>MRGSHHHHHHGIDHMPVEGSEEDKSQTGVNRASKGGLIYGNYLHLEKVLNAQELQSETKGNKIHDEHLFIITHQAYELWFKQILWELDSVREIFQNGHVRDERNMLKVVSRMHRVSVILKLLVQQFSILETMTALDFNDFREYLSPASGFQSLQFRLLENKIGVLQNMRVPYNRRHYRDNFKGEENELLLKSEQEKTLLELVEAWLERTPGLEPHGFNFWGKLEKNITRGLEEEFIRIQAKEESEEKEEQVAEFQKQKEVLLSLFDEKRHEHLLSKGERRLSYRALQGALMIYFYREEPRFQVPFQLLTSLMDIDSLMTKWRYNHVCMVHRMLGSKAGTGGSSGYHYLRSTVSDRYKVFVDLFNLSTYLIPRHWIP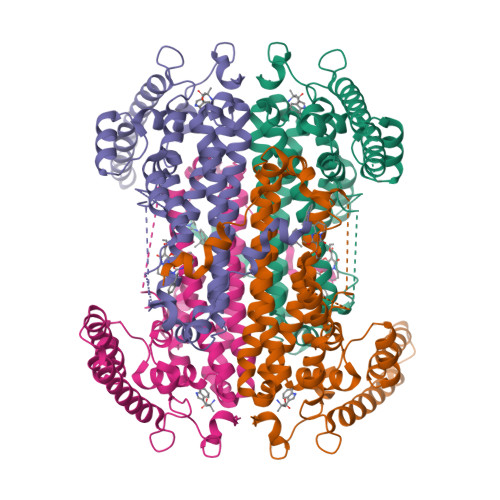KMNPTIHKFLYTAEYCDSSYFSSDESD[4x]>SNAERKEGEVAGLDMNISQFLKSLGLEHLRDIFETEQITLRVLADMGHEELKEIGI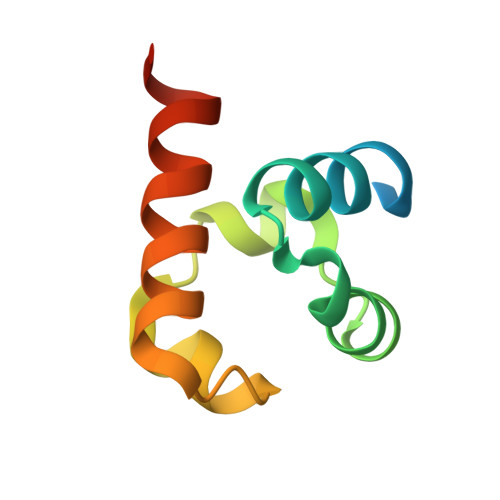NAYGHRHKLIKGVERLLGGQQGT[6x]>XLKKLCKLLKKLCKL[24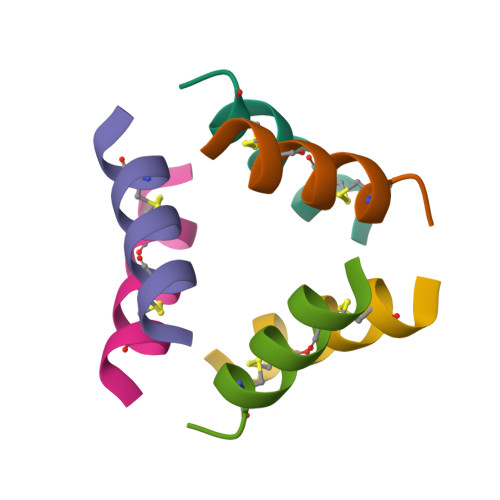x]>MKTVVFAYHDMGCLGIEALLAAGYEISAIFTHTDNPGEKAFYGSVARLAAERGIPVYAPDNVNHPLWVERIAQLSPDVIFSFYYRHLIYDEILQL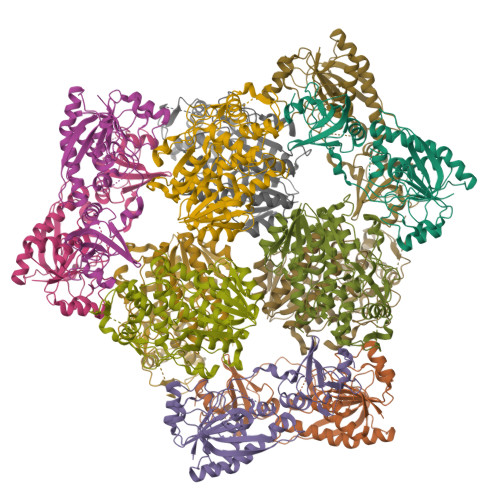APAGAFNLHGSLLPKYRGRAPLNWVLVNGETETGVTLHRMVKRADAGAIVAQLRIAIAPDDIAITLHHKLCHAARQLLEQTLPAIKHGNILEIAQRENEATCFGRRTPDDSFLEWHKPASVLHNMVRAVADPWPGAFSYVGNQKFTVWSSRVHPHASKAQPGSVISVAPLLIACGDGALEIVTGQAGDGITMQGSQLAQTLGLVQ[6x];>[6x]MRVLILGVNGFIGNHLTERLLREDHYEVYGLDIGSDAISRFLNHPHFHFVEGDISIHSEWIEYHVKKCDVVLPLVAIATPIEYTRNPLRVFELDFEENLRIIRYCVKYRKRIIFPSTSEVYGMCSDKYFDEDHSNLIVGPVNKPRWIYSVSKQLLDRVIWAYGEKEGLQFTLFRPFNWMGPRLDNLNAARIGSSRAITQLILNLVEGSPIKLIDGGKQKRCFTDIRDGIEALYRIIENAGNRCDGEIINIGNPENEASIEELGEMLLASFEKHPLRHHFPPFAGFRVVESSSYYGKGYQDVEHRKPSIRNAHRCLDWEPKIDMQETIDETLDFFLRTVDLTD>MAHHHHHHMTKRIAVV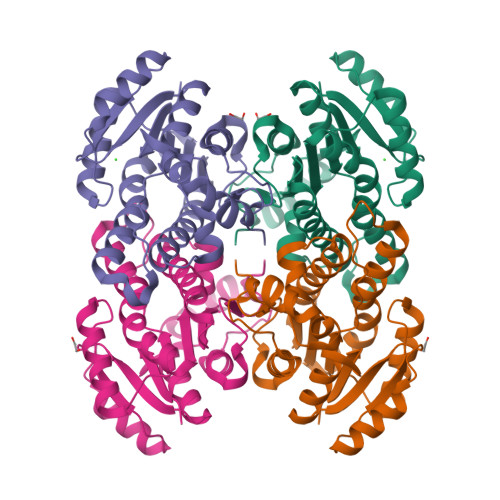TGGMGGLGEAVSIRLNDAGHRVVVTYSPNNTGADRWLTEMHAAGREFHAYPVDVADHDSCQQCIEKIVRDVGPVDILVNNAGITRDMTLRKLDKVNWDAVIRTNLDSVFNMTKPVCDGMVERGWGRIVNISSVNGSKGSVGQTNYAAAKAGMHGFTKSLALEIARKGVTVNTVSPGYLATKMVTAIPQDILDTKILPQIPAGRLGKPEEVAALVAYLCSEEAGFVTGSNIAINGGQHMH[2x]> MVMGI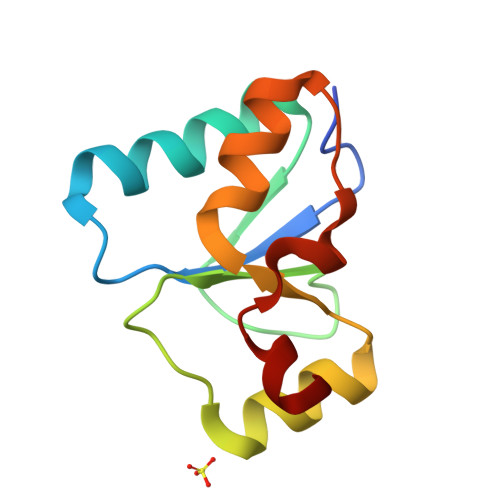FANCIFCLKVKYLPQQQKKKLQTDIKENGGKFSFSLNPQCTHIILDNADVLSQYQLNSIQKNHVHIANPDFIWKSIREKRLLDVKNYDPYKPLDI>[2x]MDIWYGTAAVPKDLDNSAVTIGVFDGVHRGHQKLINATVEKAREVGAKAIMVTFDPHPVSVFLPRRAPLGITTLAERFALAESFGIDGVLVIDFTRELSGTSPEKYVEFLLEDTLHASHVVVGANFTFGENAAGTADSLRQICQSRLTVDVIDLLDDEGVRISSTTVREFLSEGDVARANWALGRHFYVTGPVVRGAGRGGKELGFPTANQYFHDTVALPADGVYAGWLTILPTEAPVSGNMEPEV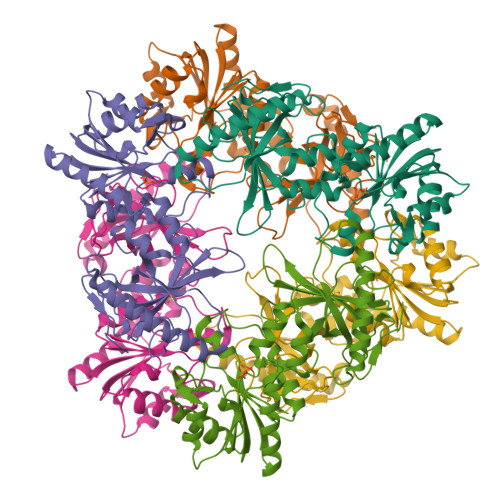AYAAAISVGTNPTFGDEQRSVESFVLDRDADLYGHDVKVEFVDHVRAMEKFDSVEQLLEVMAKDVQKTRTLLAQDVQAHKMAPETYFLQAES> MGSHHHHHHHHHHSSGHLEVLFQGPSHMVDQATLDKLEAGFKKLQDATDCKSLLKKYLNREVFDQCKSLKTALGATLLDCIQSGVENLDSGVGIYAPDAEAYTLFAPIFNPIIEDYHEGFKPTDKHPPTDFGDINTIVNVDPSGKYVVSTHVRCGRSLKGYPFNPCLTEANYKEMEDKVSAIFGTFEGELKGKYYPLTGMDKATQQQLIDDHFLFKEGDRFLQAANACRYWPTGRGIYHNDAKTFLVWVNEEDHLRIISMQKGGDLKTIFQRLVNAVNTIESKLPFSRDDRLGFLTFCPTNLGTTIRASVHIALPKLAKDKKQLEAIAAKFNLQVRGTRGEHTESEGGVYDISNKRRMGLTEYQAVKEMQDGILEMIKMEEAAP

In this work, we sequenced, cloned and overexpressed a spider arginine kinase (PpAK), an enzyme crucial for rapid energy energy fluxes in invertebrates. AK has a similar function to creatine kinase (CK) from vertebrates (ATP: N-creatine phosphotransferase, EC 2.7.3.2,) providing fast energy during muscular contraction by the back-phosphorylation of ADP by phospho-arginine. In AKs and in phosphagen kinases in general, the canonical fold is comprised of two domains; a small N-terminal globular domain and a large C-terminal α-β domain. Interestingly, the active site is located between both domains and a large conformational change occurs during catalysis as a hinged rotation (Zhou, Ellington & Chapman, 2000).

Besides the biochemical characterization, we obtained the crystallographic structures of PpAK in substrate-free from (apo-Pp-AK) and in a binary complex with the guanidino group substrate-arginine (Arg-PpAK) at 2.1 and 2.0 Å resolution, respectively. The structure of substrate-bound PpAK was obtained by soaking crystals of the apoAK in 20 mM arginine dissolved in the crystallization solution. Using a Polder map, which is an omit map where the bulk solvent is excluded during calculations, generated a much better electron density that supports modeling L-arginine into the active site and the interactions with PpAK side chains. Arg-PpAK binary complex was found is the open conformation similar to the free substrate PpAK model. Superposition of both structures do not show overall conformational changes upon arginine binding (RMSD = 0.36 Å for C-α atoms). Arginine-substrate carboxylate is stabilized by hydrogen bonds to backbone Gly64, Val65 and Gly66 and the hydroxyl group of Tyr68 to arginine amino group. The guanidino group of the arginine substrate has specific contacts in the active site. A salt bridge with Glu225 and a hydrogen bond with Cys271 position the substrate in a region with poor density. Comparing the apo vs. Arg-bound PpAK structures, it is observed that the Glu225 carboxylate lateral chain is slightly rotated to favour a hydrogen bond of arginine guanidino group end. In the PpAK-Arg structure we found that Glu225 is positioned in a similar way, making only one salt-bridge with NH2(ω)-1 of the arginine guanidino group end. This small local conformational change was also observed in LvAK-Arg structure and it is postulated to lead to a productive active site in the closed conformation.> GHMTHYKFYEAN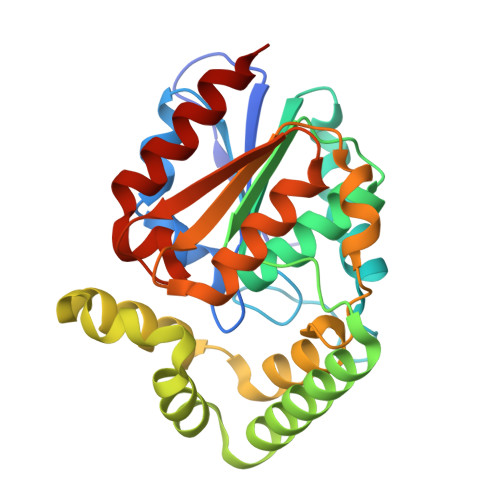VETNQVLVFLHGFLSDSRTYHNHIEKFTDNYHVITIDLPGHGEDQSSMDETWNFDYITTLLDRILDKYKDKSITLFGYSMGGRVALYYAINGHIPISNLILESTSPGIKEEANQLERRLVDDARAKVLDIAGIELFVNDWEKLPLFQSQLELPVEIQHQIRQQRLSQSPHKMAKALRDYGTGQMPNLWPRLKEIKVPTLILAGEYDEKFVQIAKKMANLIPNSKCKLISATGHTIHVEDSDEFDTMILGFLKEEQND> MLGILNKMFDPTKRTLNRYEKIANDIDAIRGDYENLSDDALKHKTIEFKERLEKGATTDDLLVEAFAVVREASRRVTGMFPFKVQLMGGVALHDGNIAEMKTGEGKTLTSTLPVYLNALTGKGVHVVTVNEYLASRDAEQMGKIFEFLGLTVGLNLNSMSKDEKREAYAADITYSTNNELGFDYLRDNMVLYKEQMVQRPLHFAVIDEVDSILIDEARTPLIISGQAAKSTKLYVQANAFVRTLKAEKDYTYDIKTKAVQLTEEGMTKAEKAFGIDNLFDVKHVAL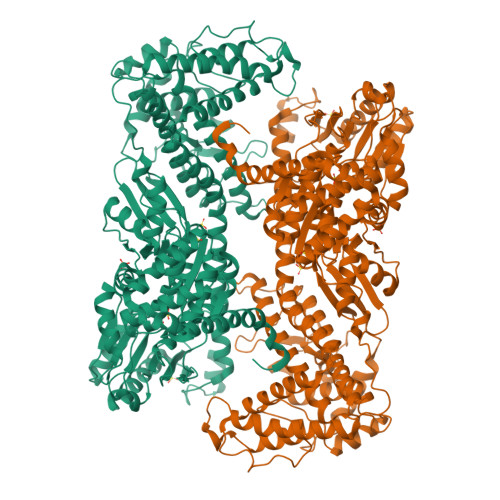NHHINQALKAHVAMQKDVDYVVEDGQVVIVDSFTGRLMKGRRYSEGLHQAIEAKEGLEIQNESMTLATITFQNYFRMYEKLAGMTGTAKTEEEEFRNIYNMQVVTIPTNRPVVRDDRPDLIYRTMEGKFKAVAEDVAQRYMTGQPVLVGTVAVETSELISKLLKNKGIPHQVLNAKNHEREAQIIEEAGQKGAVTIATNMAGRGTDIKLGEGVKELGGLAVVGTERHESRRIDNQLRGRSGRQGDPGITQFYLSMEDELMRRFGAERTMAMLDRFGMDDSTPIQSKMVSRAVESSQKRVEGNNFDSRKQLLQYDDVLRQQREVIYKQRFEVIDSENLREIVENMIKSSLERAIAAYTPREELPEEWKLDGLVDLINTTYLDEGALEKSDIFGKEPDEMLELIMDRIITKYNEKEEQFGKEQMREFEKVIVLRAVDSKWMDHIDAMDQLRQGIHLRAYAQTNPLREYQMEGFAMFEHMIESIEDEVAKFVMKAEIENNLEREEVVQGQTTAHQPQEG> MSLANRIRLHIWGDYACFTRPEMKVERVSYDVITPSAARGILSAIHWKPAINWVIDKIYVLKPIRFESVRRNELGAKISESKVSGAMKRKSVADLYTVIEDDRQQRA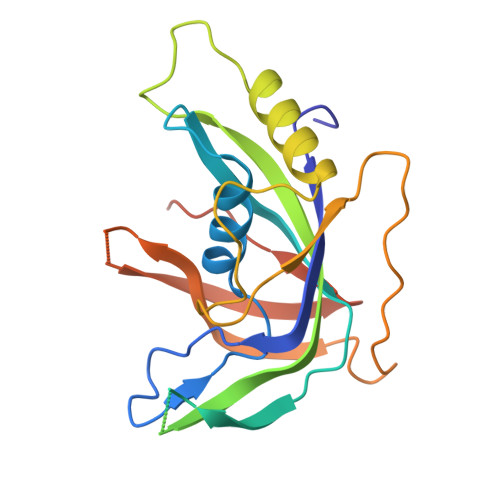ATVLKDVAYVIEAHAVMTSKAGVDENTTKHIEMFKRRALKGQCFQQPCMGVREFPAHFALIDDNDPLPLSQLSESEFNRDLGWMLHDIDFEHGNTPHFFRAELKNGVIDVPPFYAEEVKREGHHHHHH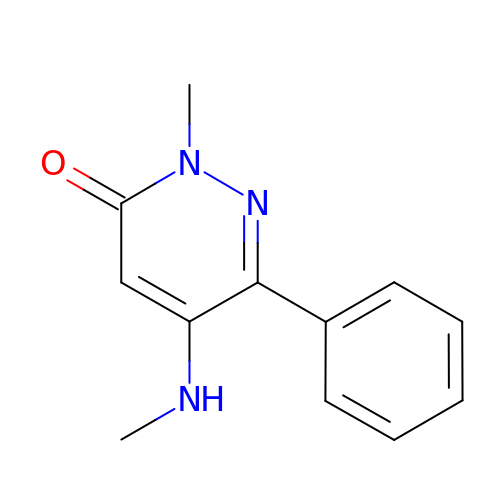2-methyl-5-(methylamino)-6-phenylpyridazin-3(2H)-one | C12 H13 N3 O | ZRCCUVSDZQJQEX-UHFFFAOYSA-N>INDPAKSAAPYHDEFPLFRSANMASPDKLSTGIGFHSFRIPAVVRTTTGRILAFAEGRRHTNQDFGDINLVYKRTKTTANNGASPSDWEPLREVVGSGAGTWGNPTPVV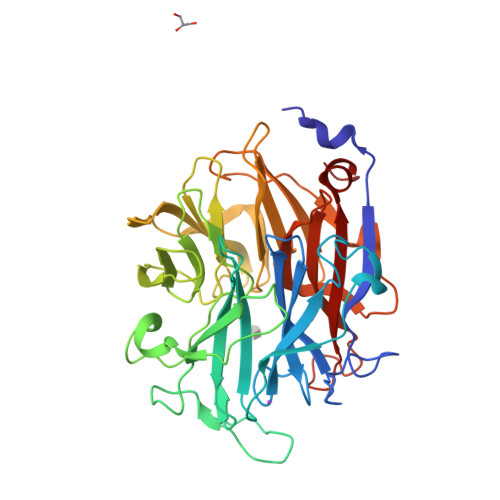DDDNTIYLFLSWNGATYSQNGKDVLPDGTVTKKIDSTWEGRRHLYLTESRDDGNTWSKPVDLTKELTPDGWAWDAVGPGNGIRLTTGELVIPAMGRNIIGRGAPGNRTWSVQRLSGAGAEGTIVQTPDGKLYRNDRPSQKGYRMVARGTLEGFGAFAPDAGLPDPACQGSVLRYNSDAPARTIFLNSASGTSRRAMRVRISYDADAKKFNYGRKLEDAKVSGAGHEGGYSSMTKTGDYKIGALVESDFFNDGTGKNSYRAIIWRRFNLSWILNGPNN[2x]> MSDNDELQQIAHLRREYTKGGLRRRDLPADPLTLFERWLSQACEAKLADPTAMVVATVDEHGQPYQRIVLLIHYDEKGMVFYTNLGSRKAHQIENNPRVSLLFPWHTLERQVMVIGKAERLSTLEVMKFFHSLPRDSQIGAWVSKQSSRISARGILESKFLELKQKFQQGEVPLPSFWGGFRVSLEQIEFWQGGEHRLADRFLYQRENDAWKIDRLAP

In Escherichia coli, PLP formation is catalyzed by pyridoxine 5’-phosphate oxidase (PNPO), a homodimeric FMN-dependent enzyme that is responsible for the last step of PLP biosynthesis and is also involved in the PLP salvage pathway. By using FMN as cofactor, PNPO catalyzes the oxidation of both pyridoxine 5’-phosphate (PNP) and pyridoxamine 5’-phosphate to PLP, reducing molecular oxygen to hydrogen peroxide. We have recently demonstrated that ePNPO undergoes an allosteric feedback inhibition by PLP, through a mechanism in which binding of substrate at the active site and binding of PLP at an allosteric site negatively affect each other to a large extent. We recently showed that an ePNPO quadruple variant (K72I/Y129F/R133L/H199A; ePNPOqm), which has a drastically reduced capability to bind PNP (and therefore PLP) at the active site, is still able to bind PLP at the allosteric site.

We crystallized this quadruple variant in both the absence of PLP (ePNPOqm) in P31 2 1 space group and presence of PLP (PLP-ePNPOqm) in P61 space group. The final model of ePNPOqm was refined to 1.56 Å resolution; the asymmetric unit contains a 212-residue subunit (residues 7–218; the entire polypeptide chain is made by 218 residues), one FMN molecule, two sulphate ions, one phosphate ion, and 174 water molecules. The second subunit of the dimer was generated by the crystallographic 2-fold axis. The quadruple mutant conserves the structural elements of the wildtype protein: five alpha helices, numbered from H1 to H5, and ten β strands. In addition, in the PLP-free ePNPOqm the N-terminal region is also visible, folded in an additional α helix (H0, residues 5–18). The β sheets core region is flanked by H1 (and H0 in PLP-free ePNPOqm) on one side and H2 on the opposite side. In this structure of ePNPOqm without PLP, the interactions between two key residues of H5 (subunit A; Arg153 and Glu157) and residues Glu195, Leu198, and Asp200 placed on the 192 to 200 helix (subunit B) are particularly important to maintain these structural elements linked together and correctly folded. In the ePNPOqm structure, the Arg197 displays a position similar to that of the wildtype protein. No PLP is present at the active site of either structures, although PLP-ePNPOqm was crystallized in the presence of excess PLP (see Experimental procedures section for details); this is evidently a consequence of the engineered active site variants.> VAKLVFFAGAAIIG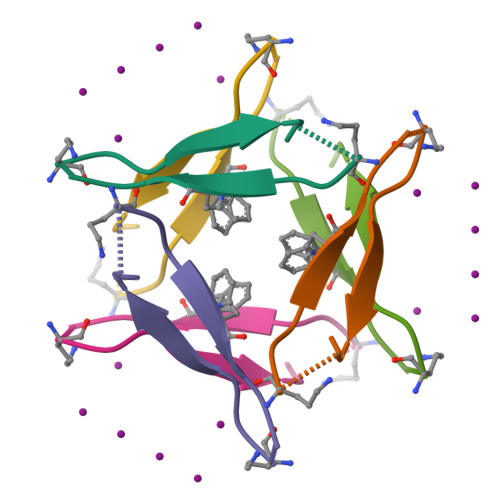LM> GSPEFMIGEEVPSDQYYWAPLAQHERGSLASLDSLRKGGP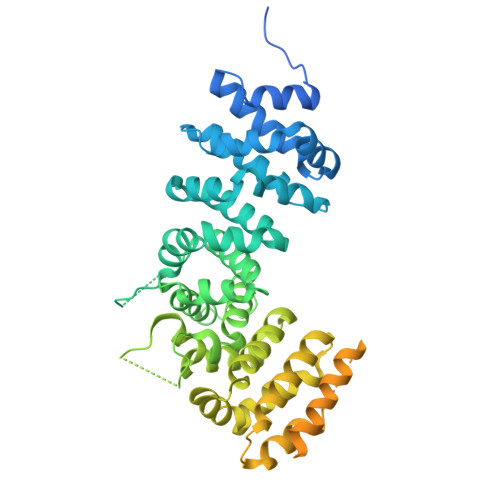PPPNWRQPELPEVIAMLGFRLDAVKSNAAAYLQHLCYRNDKVKTDVRKLKGIPVLVGLLDHPKKEVHLGACGALKNISFGRDQDNKIAIKNCDGVPALVRLLRKARDMDLTEVITGTLWNLSSHDSIKMEIVDHALHALTDEVIIPHSGWEREPNEDCKPRHIEWESVLTNTAGCLRNVSSERSEARRKLRECDGLVDALIFIVQAEIGQKDSDSKLVENCVCLLRNLSYQVHREIPQAERYQEAAPNVANNTGTSPARGYELLFQPEVVRIYISLLKESKTPAILEASAGAIQNLCAGRWTYGRYIRSALRQEKALSAIADLLTNEHERVVKAASGALRNLAVDARNKELIGKHAIPNLVKNLPGGQQNSSWNFSEDTVISILNTINEVIAENLEAAKKLRETQGIEKLVLINKSGNRSEKEVRAAALVLQTIWGYKELRKPLEKEGWKKSDFQVNLNNASRSQSSHSYDDSTLPLIDRNQKSDKKPDREEIQMSNMGSNTKSLDNNYSTPNERGDHNRTLDRSGDLGDMEPLKGTTPLMQKI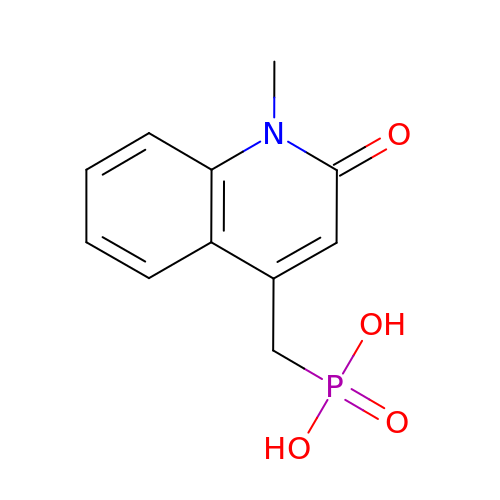[(1-methyl-2-oxo-1,2-dihydroquinolin-4-yl)methyl]phosphonic acid | C11 H12 N O4 P | LOQZOOPJJBKDAA-UHFFFAOYSA-N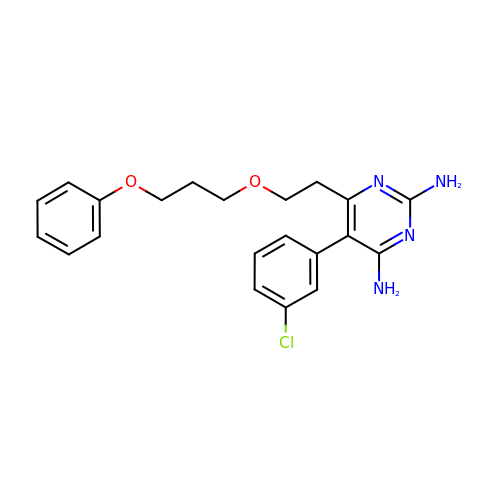5-(3-chlorophenyl)-6-[2-(3-phenoxypropoxy)ethyl]pyrimidine-2,4-diamine | C21 H23 Cl N4 O2 | CRGQDUYGPMHVEY-UHFFFAOYSA-N> MADKELKFLVVDDFSTMRRIVRNLLKELGFNNVEEAEDGVDALNKLQAGGFGFIISD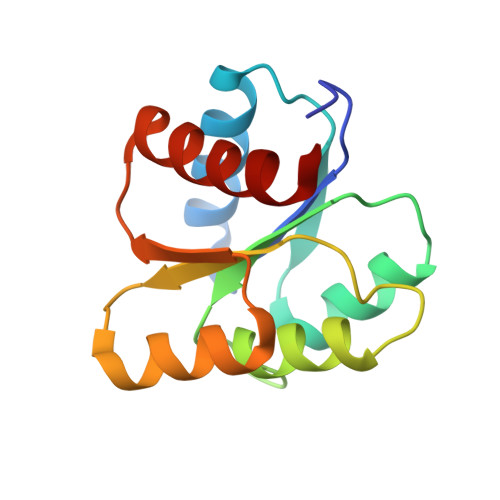WNMPNMDGLELLKTIRADSAMSALPVLMVTAEAKKENIIAAAQAGASGYVVKPFTAATLEEKLNKIFEKLGM Nine new crystal structures of CG-rich DNA 18-mers with the sequence 5′-GGTGGGGGC-XZ-GCCCCACC-3′, which are related to the bacterial repetitive extragenic palindromes, are reported. All 18-mers crystallized as isomorphic tetragonal crystals with one strand of a right-handed antiparallel duplex in the asymmetric unit. All reported structures co-crystallized with the Sr2+ cation located between nucleotides 6 and 7 and (by symmetry) 12 and 13.

Two of the four YR and RY variants unable to form Watson–Crick pairs were crystallized, Chom-18-AC and Chom-18-GT, but their base-pairing topology was not assigned. NtC classes provided valuable help with building the initial models of six of the nine 18-mers, i.e. Chom-18-AT, Chom-18-CG, Chom-18-GC, Chom-18-GT, Chom-18-TC and Chom-18-AG. When we measure the distances between the C1′ atom of nucleotide 9 and C1′ of its symmetry-related base-paired nucleotide 10 in all 18-mers, the order from the shortest to the longest is TT (7.9 Å) < CC < TC < GT < GC < AC < AT < TA < CG < AG (12.1 Å). This trend follows the size of the pyrimidine–pyrimidine (Y–Y), pyrimidine–purine (Y–R/R–Y) and purine–purine (R–R) pairs regardless of the type of base pair involved.

> GGTGGGGCGTGCCCCACC>GSMASTQDAVHTDAVQDWKNGTINAQLTLDLARARMRLPADRTAASQFLRYKAPAQLKDVYLSVLVDSQNRVGDCLAHEKIRLADITALVDAGHHAVTTLSPSVRSLQLSHQTPLTALARLFVTHETAYVPAIPPTSAVSRPYTGILIDARGSLPVHGEYVSEPLSACLFPKIWSTDMDLIYEKNMVHPDRAKAWGVVRYGSVWDEKMYRDRIGTTPLKIIARGVFGQQRTDPIIASKDAAQIL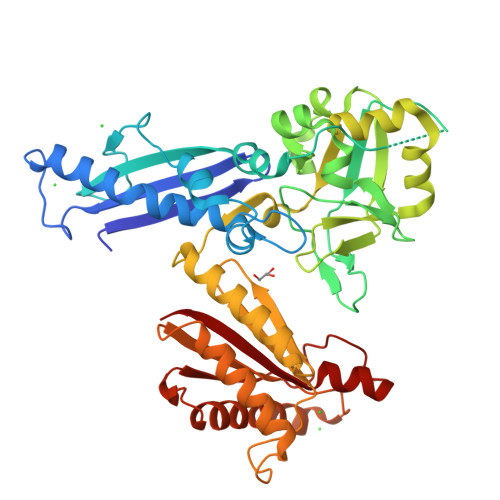ARPENLRLLAEGNVIILCDEAALRVHVPYPLVDEHFYFAYHDVKRFLTDERSPGVGVRSGINTLKITVYDVRFVANSPEILASEKDRVDVIATALKKMGPYTRFLIEGHTADLHRPQEEAALSVARAQRMAQELSRRGIEMTRITTAGHGATKPIAPSDTHANKAKNRRVEITILRD[2x]5-(4-azanylbutyl)-3-pentyl-quinolin-2-amine | C18 H27 N3 | 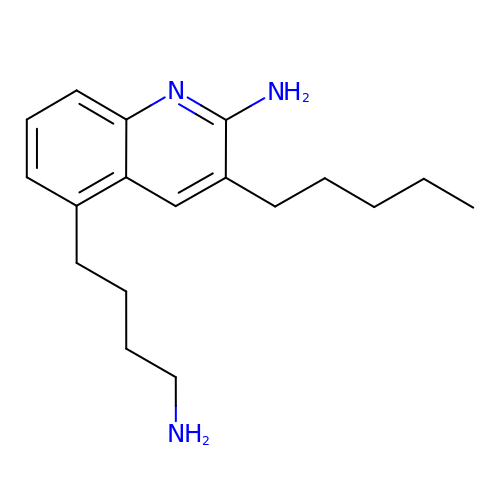GHXJTPWIBLPAON-UHFFFAOYSA-N>MTRKQATIAVRSGLNDDEQYGCVVPPIHLSSTYNFTGFNEPRAHDYSRRGNPTRDVVQRALAELEGGAGAVLTNTGMSAIHLVTTVFLKPGDLLVAPHDCYGGSYRLFDSLAKRGCYRVLFVDQGDEQALRAALAEKPKLVLVESPSNPLLRVVDIAKICHLAREVGAVSVVDNTFLSPALQNPLALGADLVLHSCTKYLNGHSDVVAGVVIAKDPDVVTELAWWANNIGVTGGAFDSYLLLRGLRTLVPRMELAQRNAQAIVKYLQTQPLVKKLYHPSLPENQGHEIAARQQKGFGAMLSFELDGDEQTLRRFLGGLSLFTLAE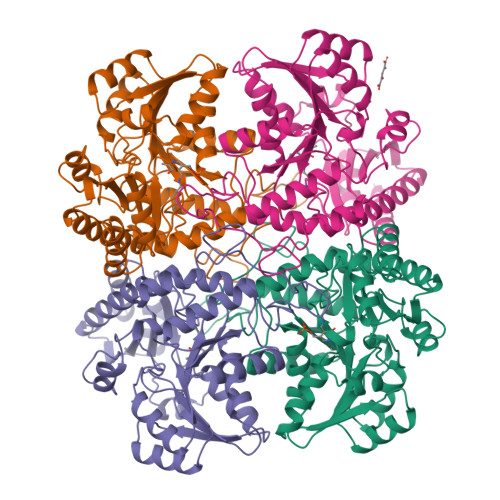SLGGVESLISHAATMTHAGMAPEARAAAGISETLLRISTGIEDGEDLIADLENGFRAANKG[4x]The two gel-forming mucins MUC5AC and MUC5B constitute the main structural components of the mucus protecting the underlying epithelia in the respiratory system. The VWD assemblies are formed by the VWD domain, C8, trypsin inhibitor like (TIL) and E domains, except the VWD’ domain that only has the TIL and E domains. We determined the cryoEM structures of the wild type D3 assembly of the human MUC5AC mucin and the structural single nucleotide polymorphisms (SNP) variants Arg996Gln and Arg1201Trp that affect intermolecular interactions. The D3 assembly forms covalent dimers that can appear in two alternative conformations, open and closed, where the closed conformation dimers interact through an arginine-rich loop in the TIL3 domain to form tetramers.

The Arg1201Trp SNP, frequent in European population, shows a double role in the conformation alteration of the VWD3 assembly. In contrast, the Arg1201Trp mutation, placed in the β1-β2 TIL3 loop, only affects the adjacent residues. The solvent exposed arginine is substituted by a tryptophan pointing toward the VWD-C8/TIL interface. The tryptophan accommodates into the VWD3 hydrophobic interfacing region in close proximity to Leu1013. The Arg1201Trp mutation implied a more discrete reduction in open conformation particles showing a ratio of 89:11 between the closed and open conformation. However, it represents a reduction of 35% respect to the WT. In the closed conformation it establishes a novel interaction between the TIL3 domain and VWD3, and the open conformation removes the possibility of a putative salt bridge between Arg1201 and Glu981. By that we can speculate that this mutation should favor the closed conformation, even though open conformation molecules were observed in cryoEM. On the other hand, the presence of the tryptophan interacting with VWD3 could affect the TIL3 flexibility important for the interaction. Nevertheless, we found that the Arg1201Trp SNP could favor tetramerization and thus net-like formation.

>[2x]DAAQPARRAVRSSRHHHHHHGSATCAVYGDGHYLTFDGQSYSFNGDCEYTLVQNHCGGKDSTQDSFRVVTENVPCGTTGTTCSKAIKIFLGGFELKLSHGKVEVIGTDESQEVPYTIRQMGIYLVVDTDIGLVLLWDKKTSIFINLSPEFKGRVCGLCGNFDDIAVNDFATRSRSVVGDVLEFGNSWKLSPSCPDALAPKDPCTANPFRKSWAQKQCSILHGPTFAACHAHVEPARYYEACVNDACACDSGGDCECFCTAVAAYAQACHEVGLCVSWRTPSICPLFCDYYNPEGQCEWHYQPCGVPCLRTCRNPRGDCLRDVWGLEGCYPKCPPEAPIFDEDKMQCVATCPTPPLPPRCHVHGKSYRPGAVVPSDKNCQSCLCTERGVECTYKAEACVCTYNGQRFHPGDVIYHTTDGTGGCISARCGANGTIERRVYPCSPTTPVPPTTFSFSTPPLVVSSTHTPSNGPSSAHTGPPSSAWPTTAGTDDDDKTSEQKLISEEDLSRKLTR>[2x]MADYKDDDDKGTDYKDDDDKLEVLFQGPMEANQCPLVVEPSYPDLVINVGEVTLGEENRKKLQKIQRDQEKERVMRAACALLNSGGGVIRMAKKVEHPVEMGLDLEQSLRELIQSSDLQAFFETKQQGRCFYIFVKSWSSGPFPEDRSVKPRLCSLSSSLYRRSETSVRSMDSREAFCFLKTKRKPKILEEGPFHKIHKGVYQELPNSDPADPNSDPADLIFQKDYLEYGEILPFPASQLVEFKQFSTKHFQEYVKRTIPEYVPAFANTGGGYLFIGVDDKSREVLGCAKENVDPDSLRRKIEQAIYKLPCVHFCQPQRPITFTLKIVNVLKRGELYGYACMIRVNPFCCAVFSEAPNSWIVEDKYVCSLTTEKWVGMMTDTDPDLLQLSEDFECQLSLSSGPPLSRPVYSKKGLEHKKELQQLLFSVPPGYLRYTPESLWRDLISEHRGLEELINKQMQPFFRGILIFSRSWAVDLNLQEKPGVICDALLIAQNSTPILYTILREQDAEGQDYCTRTAFTLKQKLVNMGGYTGKVCVRAKVLCLSPESSAEALEAAVSPMDYPASYSLAGTQHMEALLQSLVIVLLGFRSLLSDQLGCEVLNLLTAQQYEIFSRSLRKNRELFVHGLPGSGKTIMAMKIMEKIRNVFHCEAHRILYVCENQPLRNFISDRNICRAETRKTFLRENFEHIQHIVIDEAQNFRTEDGDWYGKAKSITRRAKGGPGILWIFLDYFQTSHLDCSGLPPLSDQYPREELTRIVRNADPIAKYLQKEMQVIRSNPSFNIPTGCLEVFPEAEWSQGVQGTLRIKKYLTVEQIMTCVADTCRRFFDRGYSPKDVAVLVSTAKEVEHYKYELLKAMRKKRVVQLSDACDMLGDHIVLDSVRRFSGLERSIVFGIHPRTADPAILPNVLICLASRAKQHLYIFPWGGH

Schlafen 11 (SLFN11) is an interferon-inducible antiviral restriction factor with tRNA endoribonuclease and DNA binding functions. It is recruited to stalled replication forks in response to replication stress and inhibits replication of certain viruses such as the human immunodeficiency virus 1 (HIV-1) by modulating the tRNA pool. SLFN11 consists of an N-terminal endonuclease domain (residues 1–353), termed Slfn core domain, followed by a linker domain (residues 354–576) and a C-terminal domain with homology to superfamily I (SF I) DNA/RNA helicases (residues 577–901). SLFN11 forms a homodimer with the helicase domains adopting an autoinhibited conformation.

We recorded datasets of SLFN11wt and SLFN11E209A and 2D classifications yielded classes of monomeric as well as C2 symmetric dimeric SLFN11. Furthermore, monomeric and dimeric SLFN11E209A were reconstructed from two different datasets, resulting in maps with global resolutions of 4.0 Å and 3.25 Å, respectively. In the apoenzyme structure additional density for a metal ion appears at the proposed nuclease active site which is coordinated by residues E209 and E214. Density for a metal ion could not be observed in the cryo-EM map of mutant SLFN11E209A. Mutation of the ion coordinating residues (E209A, E214A) abolished the nuclease activity completely. The active site residues E209, E214 and K216 are essential for catalysis.> MSNGDGLIRSLVDGDLEGFRQGFESFLDQCPSFLYHVSAGRFLPVFFFSMFSTAHDANILNANERVYFRFDNHGVNPRNGENRNTANLKVAVYRDGQQVVRCYSISDRPNSDGLRFSTRERNALVQEIRRQNPNLREEDLNFEQYKVCMHGKGKSQGEAIATVFEVIREKDRQGRDKFAKYSASEVHFLRQLFRNHRLTIKEIEGRQLNQNQLRQLGRSVNFTRVEPGQQRIDNFMEMLASNQRQDVRDSLRGDILEYVTDTYNNYRAQIENNIEGRSQKFESHGFLLGFLANFSHRYTIGVDLDLSPRNSHVAFLVRHQVERENIPIVINLATRAPPYIALNRARSHAERLHVFSFIPIHTESRNTVCVGLNFNLNLDPFSVDTVGLQQDRFPLVQRLFECLENEGIRENIRDFLLHHLPAEIPRNAENYDRIFDCITGFAFGNSAFDRHPLELEEEDEAPITKYIFRHGDEGLRCLTMVFHAEGSDIVILHIRAHDAQQQGAINLQTLNVNGNDVHVWEVSCTLNNQLELDIDLPNDLGLYHDYQNNNANNFLAGDLVQVPNTENVHNTLNQVVNDGWKNIAQHRGLFQEISGALMPLVDTINVNSEDKFRSILHGTFYASDNPYKVLAMYKVGQTYSLKRGQEEEGERVILTRITEQRLDLLLLRQPRENDLDTHPIGYVLRLANNAEEVGQQQNDARQEIGRLKKQHRGFIPITSGNEVVLFPIVFNRDAHEAGNLI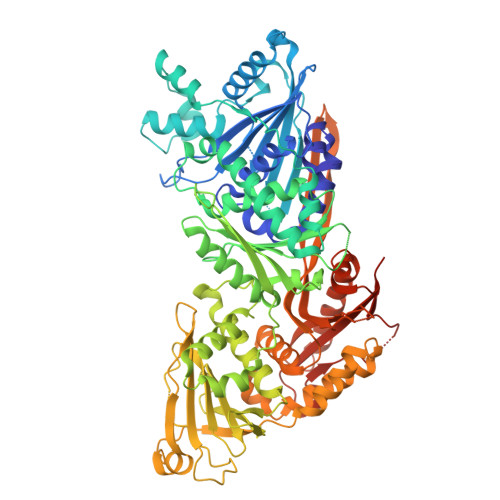LFPEGIGREEHVHRLDRHVRLEHHHHHH N-{4-[4-(2-amino-4-oxo-4,7-dihydro-3H-pyrrolo[2,3-d]pyrimidin-6-yl)butyl]benzoyl}-L-glutamic 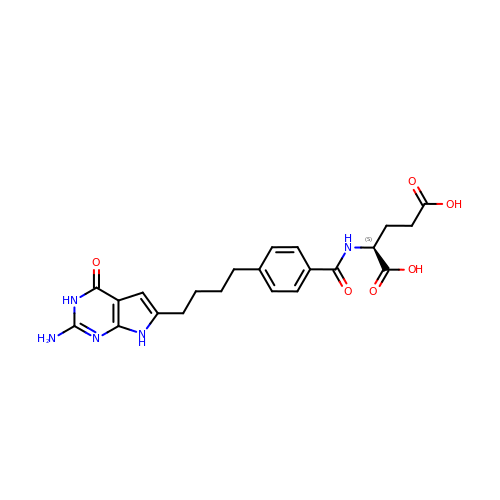acid | C22 H25 N5 O6 | CEPQCJFDTGQKDN-INIZCTEOSA-N>[2x]STGAANKSLSLLST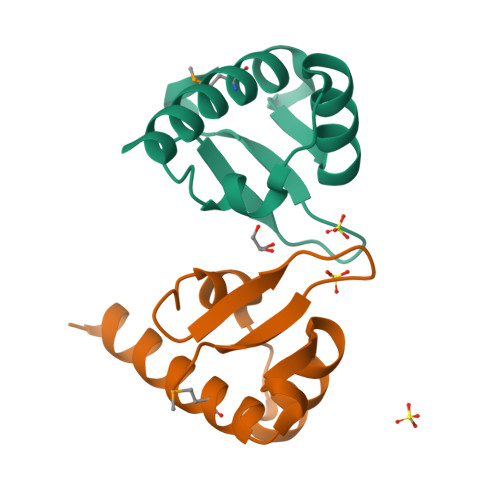ETMSILQDAPACCLPLFKFIDIYEKKYGHKLNVSDLYKLTDTIAIREQGNGRLVCLLPSNQ> SHMQSRELKTVSADCKKEAIEKCAQWVVRDCRPFSAVSGSGFIDMIKFFIKVKAEYGEHVNVEELLPSPITLSRKVTSDAKEKKALIGREIKSAVEKDGASATIDLWTDNYIKRNFLGVTLHYHENNELRDLILGLKSLDFERSTAENIYKKLKAIFSQFNVEDLSSIKFVTDRGANVVKSLANNIRINCSSHLLSNVLENSFEETPELNMPILACKNIVKYFKKANLQHRLRSSLKSECPTRWNSTYTMLRSILDNWESVIQILSEAGETQRIVHINKSIIQTMVNILDGFERIFKELQTCSSPSLCFVVPSILKVKEICSPDVGDVADIAKLKVNIIKNVRIIWEENLSIWHYTAFFFYPPALHMQQEKVAQIKEFCLSKMED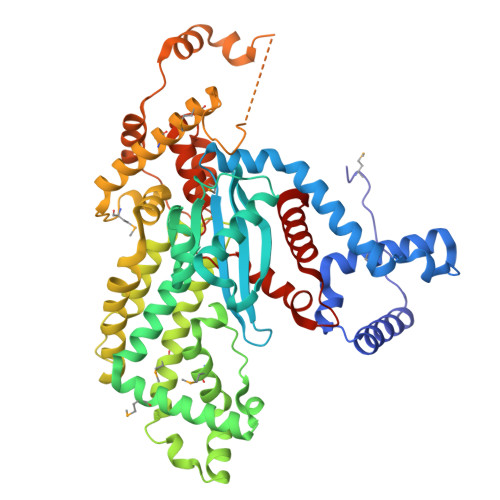LELINRMSSFNELSATQLNQSDSNSHNSIDLTSHSKDISTTSFFFPQLTQNNSREPPVCPSDEFEFYRKEIVILSEDFKVMEWWNLNSKKYPKLSKLALSLLSIPASSAASERTFSLAGNIITEKRNRIGQQTVDSLLFLNSFYKNFCK>[4x]K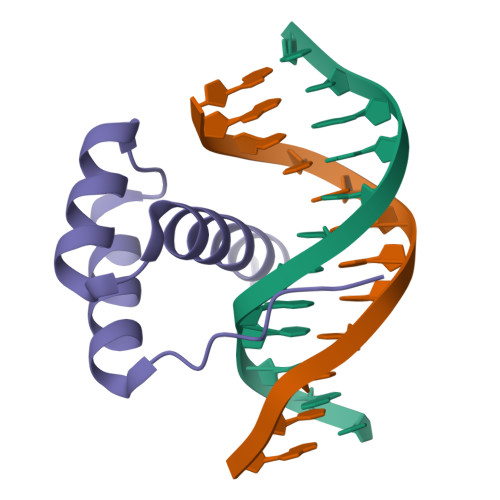PRKARTAFSDHQLNQLERSFERQKYLSVQDRMDLAAALNLTDTQVKTWYQNRRTKWKRQTA>MILFRKFRVLILTVFLIACTMHIMIDLLPKLEKRAAGSSSSAGGGSGCSCAHTPGEEPRSWGKQRARAADPGWPNKHSLRLLQDFSNEPNSNLTSQSREKVTERAGSEKQGSGKRGLMREADSRQRRTDVRVSSVLQSLFEHPLYRTVLPDLTEEDTLFNLNAEIRLYPKAAGQQEWHNEGNVEEEEFSPPGEANSESYPNWLRFHIGINRYELYSRHNPVIAALLRDLLSQKISSVGMKSGGTQLKLIMSFQNYGQALFKPMKQTREQETPPDFFYFSDFERHNAEIAAFHLDRILDFRRVPPVAGRLVNMTREIRDVTRDKKLWRTFFVSPANNICFYGECSYYCSTEHALCGKPDQIEGSLAAFLPDLALAKRKTWRNPWRRSYHKRKKAEWEVDPDYCDEVKQTPPYDRGTRLLDIMDMTIFDFLMGNMDRHHYETFEKFGNDTFIIHLDNGRGFGKHSHDEMSILVPLTQCCRVKRSTYLRLQLLAKEEYKLSSLMEESLLQDRLVPVLIKPHLEALDRRLRLVLKVLSDCVEKDGFSAVVENDLDGQPSVHGGR[12x]

The Fam20 proteins are recently identified kinases that regulate essential cellular processes by phosphorylating proteins and proteoglycans. The human genome encodes three Fam20 paralogs: Fam20A, Fam20B, and Fam20C13. Remarkably, each has a distinct biochemical activity. Here, we use a combination of structural biology, biochemistry, and phylogenetics to elucidate the molecular functions and evolutionary relationships of the three Fam20 kinases.

The human Fam20C protein crystallized but the crystals diffracted poorly. To gain structural insights into the Fam20C homodimer, we crystallized a Fam20C ortholog from zebrafish (Danio rerio, drFam20C), which is 86% identical (94% similar) to human Fam20C in the kinase domain, and determined its structure. There are 12 molecules of drFam20C in the crystal asymmetric unit, which organizes into six pairs of homodimers similar in overall structure to the Fam20A−Fam20C heterodimer. All the residues that participate in the drFam20C dimer interface are conserved in human Fam20C, including residues corresponding to Phe299C, Phe300C, Phe354C, Pro357C, Glu374C, and His375C (Phe275, Phe276, Phe330, Pro333, Glu350, and His351 in drFam20C), mutations of which reduce Fam20C activity. These analyses, together with the biochemical results described above, suggest that the human Fam20C protein probably forms a similar homodimer, and that dimer formation is critical for allosterically activating kinase activity. A comparison of the drFam20C homodimer with the Fam20A−Fam20C heterodimer suggests that Fam20C uses an almost identical set of residues to interact with itself and Fam20A. All Fam20C structures obtained so far are involved in a homodimer configuration or heterodimer with Fam20A, and likely reflect an active conformation. Thus, we propose that the Fam20C homodimer plays a “house-keeping” function, whereas Fam20A is employed when Fam20C activity is in high demand.(2-oxo-2-{[(1s,2R,3S,4s,5R,6S)-2,3,4,5,6-pentakis(phosphonooxy)cyclohexyl]oxy}ethyl)phosphonic acid | C8 H20 O25 P6 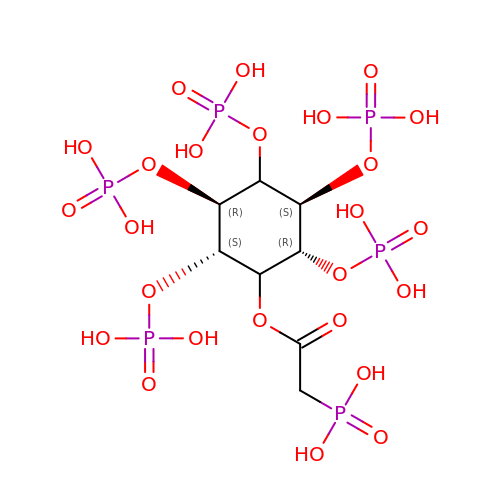| JGWVNODNEALCIO-QEEWUKHFSA-N>[2x]GPQRIVQLASRIQDACEVAGIQGDILSLVYTDARIDSAIKDELIKTLDGKILSTSELFNDFAVPLSYHEIALFIFKIADFRDHEVIMAKWDELFQSLRMEFNNTGKKEDSMNFINLLSNVLI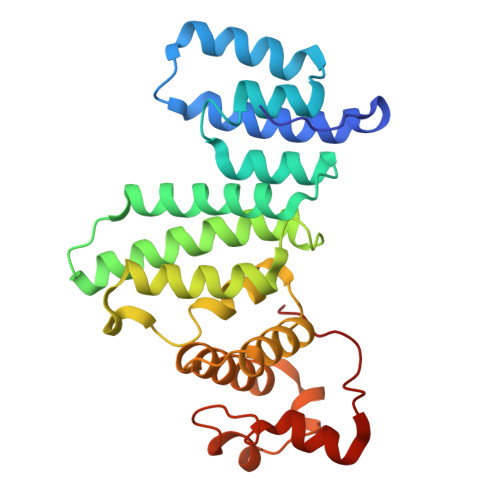KIGKNVQDSEFIFPIFELFPIVCNFFYETLPKEHIVSGSIVSIFITAGVSFNKMYYILKELIETSDSDNSVFNKEMTWLIHEWYKSDRKFRDIISYNDIIHLKEYKIDNDPIEKYVKNSGNNLGICFYKE>[2x]MSGADRSPNAGAAPDSAPGQAAVASAYQRFEPRAYLRNNYAPPRGDLCNPNGVGPWKLRCLAQTFATGEVSGRTLIDIGSGPTVYQLLSACSHFEDITMTDFLEVNRQELGRWLQEEPGAFNWSMYSQHACLIEGKGECWQDKERQLRARVKRVLPIDVHQPQPLGAGSPAPLPADALVSAF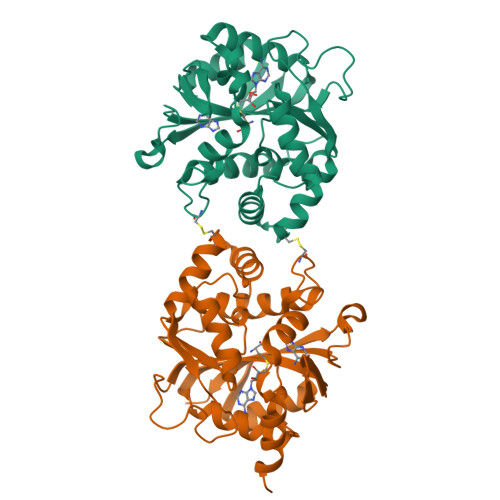CLEAVSPDLASFQRALDHITTLLRPGGHLLLIGALEESWYLAGEARLTVVPVSEEEVREALVRSGYKVRDLRTYIMPAHLQTGVDDVKGVFFAWAQKVGLEHHHHHH>GSHMEAVQNRIVEAAERVPGVRGVIHLRARYVGQDIWADMIIGVDPENTVEQAHEICEAVQAAVCGKIRRIESLHVSAEAREI[4x]

One group of metal ion efflux transporters that regulates metal ion homeostasis and can be found in all domains of life is the Cation Diffusion Facilitator (CDF) protein family. One of the most highly conserved and abundant integral MM proteins is the CDF transporter MamM. MamM was recently proposed to function as a magnetosome-directed iron transporter required for iron biomineralization since its deletion abolished magnetite biomineralization and mutation of residues within the conserved TMD metal-binding site resulted in alterations of magnetite crystal size, morphology and even mineral phase. To summarize our results we present an alternative model for the CDF CTD mode of action, in which we propose that upon metal cation binding, the CTD induces conformational changes towards a tighter and more compact fold which allows the activation of iron transport through the TMD.

Each MamM monomer (residues 215–293) adopts the metallochaperone-like typical fold of CDF CTDs whilst the C-terminal tail (residues 294–318) is disordered and could not be traced in the electron density map. To validate that the disordered C-terminal tail have no effect on the domain fold, we determined the structures of a C-terminal truncation MamM-CTD mutant (residues 215–293) that adopted a similar CTD fold. As observed previously, the decreased number of particles per cell was at least partially a consequence of a substantial number of cells within the population that remained non-magnetic (10–20%). These previous studies also revealed that transcomplementation of a truncated C-terminal tail MamM mutant also allows the formation of wild-type-like particle. ITC measurements of the CTD single point mutants and the C-terminal truncation mutant revealed that the binding affinities remained in the same order of magnitude as the wild-type, with some alternation in the number of binding sites.>[6x]MTNKAIIHSDNAPAAIGTYSQAVKVNNTVYLSGQIPLDPVTMQLVEGDFAVQAHQVFKNLRAVCEAAGGGLRDIVKLNVYLTDLANFPIVNEVMGQYFQAPYPARAA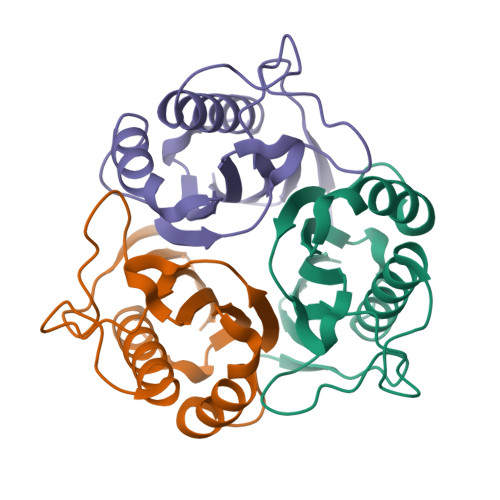IGINQLPRASLIEADGIMVI>[2x]GETPEPRTTRTILVYMMANNSLNSFASKNIESMIEGATSKNLNGGNLIVYYAPAGSPPELLRIKEENGVVKKIHLKDYEKQNSADPDVMRSVIGEVVSQYPADSYGLVLWSHGTAWLPSDYQNKLK;>AFGQDGNNWMEIDDLAKGLPDDLFDFILFDACYMASVECTYELRNKAEYILASPTETMADGWPYEEMMPQLFATDLQLEKVGETFYNHYLNNTYPYATVSLTKTSELDNLKSAIHDILADKTESDIYSLDPKNMQRLEYLYRSPGMLYDFNDYIKQLATAEQYDRFISCLDKAVVYKAHTPKSYYAAIGNALPIKSYCGLTIFVPQESLPKMLEWYKQRVGWYKAVYE[2x]

As part of an ongoing project to characterize commensal bacteria in the microbiome that inhabit the human gut, the structure of C11 peptidase, PmC11, from Parabacteroides merdae was determined using the Joint Center for Structural Genomics (JCSG)4 HTP structural biology pipeline. The crystal structure of PmC11 now provides three-dimensional information for a member of the clostripain C11 family of cysteine peptidases. The enzyme exhibits all of the key structural elements of clan CD members, but is unusual in that it has a nine-stranded central β-sheet with a novel C-terminal domain. The substrate specificity of PmC11 is Arg/Lys and the crystal structure revealed an acidic pocket for specific binding of such basic substrates.

The crystal structure of the catalytically active form of PmC11 revealed an extended caspase-like α/β/α sandwich architecture comprised of a central nine-stranded β-sheet, with an unusual C-terminal domain (CTD), starting at Lys250. A single cleavage was observed in the polypeptide chain at Lys147, where both ends of the cleavage site are fully visible and well ordered in the electron density. The two ends of the cleavage site are remarkably well ordered in the crystal structure and displaced from one another by 19.5 Å. Moreover, the C-terminal side of the cleavage site resides near the catalytic dyad with Ala148 being 4.5 and 5.7 Å from His133 and Cys179, respectively. Consequently, it appears feasible that the helix attached to Lys147 (α3) could be responsible for steric autoinhibition of PmC11 when Lys147 is covalently bonded to Ala148. Collectively, these data suggest that the pro-form of PmC11 is autoinhibited by a section of L5 blocking access to the active site, prior to intramolecular cleavage at Lys147. This cleavage subsequently allows movement of the region containing Lys147 and the active site to open up for substrate access. His133 and Cys179 were found at locations structurally homologous to the caspase catalytic dyad, and other clan CD structures, at the C termini of strands β5 and β6, respectively. The PmC11 structure reveals that the catalytic dyad forms part of a large acidic pocket, consistent with a binding site for a basic substrate. Asp177 is located near the catalytic cysteine and is conserved throughout the C11 family, suggesting it is the primary S1 binding site residue.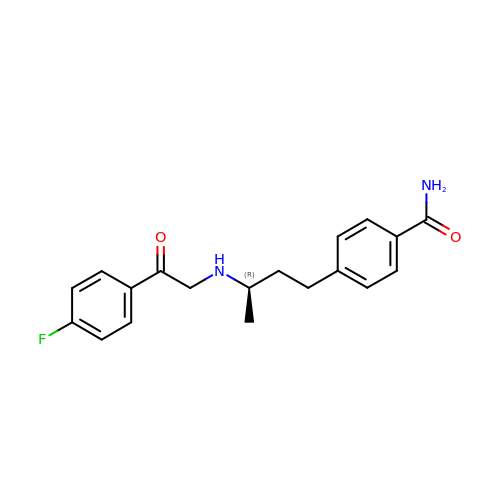4-[(3R)-3-{[2-(4-FLUOROPHENYL)-2-OXOETHYL]AMINO}BUTYL]BENZAMIDE | C19 H21 F N2 O2 | OIWWNWQZJJKBTR-CYBMUJFWSA-N>[4x]IQNQAKSV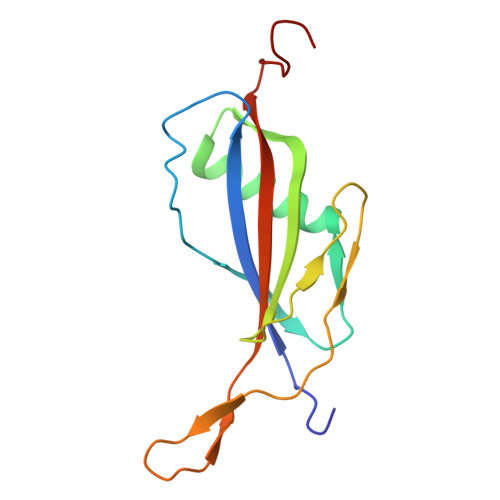DVEYTVQFTPLNPDDDFRPGLKLTKLLKTLAIGDTITSQELLAQAQSILNKNHPGYTIYERDSSIVTHDNDIFRTILPMDQEFTYRVKNREQAYRINKKSGLNEEINNTDLISEKYYVLKKGEKPYDPFD>[2x]GSYPKDKFEKINGTWYYFDSSGYMLADRWRKHTDGNWYWFDNSGEMATGWKKIADKWYYFNEEGAMKTGWVK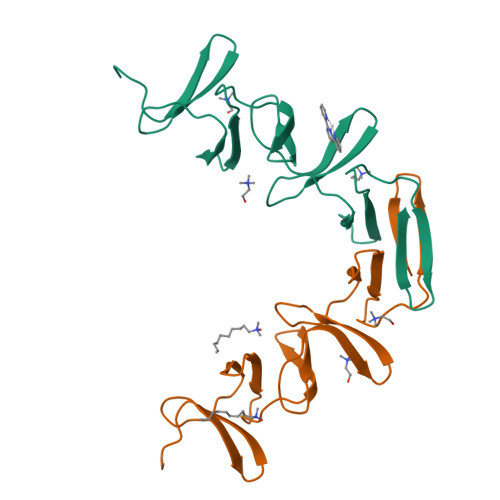YKDTWYYLDAKEGAMVSNAFIQSADGTGWYYLKPDGTLADRPEFTVEPDGLITVK> MKEVEVLMETKNTQSPQTPLVEPVTERTKLQEHTIFTQLKKNIPKTRYNRDYMLSMANIPERIINVGVIGPLHSGKTSLMDLLVIDSHKRIPDMSKNVELGWKPLRYLDNLKQEIDRGLSIKLNGSTLLCTDLESKSRMINFLDAPGHVNFMDETAVALAASDLVLIVIDVVEGVTFVVEQLIKQSIKNNVAMCFVINKLDRLILDLKLPPMDAYLKLNHIIANINSFTKGNVFSPIDNNIIFASTKLGFTFTIKEFVSYYYAHSIPSSKIDDFTTRLWGSVYYHKGNFRTKPFENVEKYPTFVEFILIPLYKIFSYALSMEKDKLKNLLRSNFRVNLSQEALQYDPQPFLKHVLQLIFRQQTGLVDAITRCYQPFELFDNKTAHLSIPGKSTPEGTLWAHVLKTVDYGGAEWSLVRIYSGLLKRGDTVRILDTSQSESRQKRQLHDISKTETSNEDEDEDDETPSCEVEEIGLLGGRYVYPVHEAHKGQIVLIKGISSAYIKSATLYSVKSKEDMKQLKFFKPLDYITEAVFKIVLQPLLPRELPKLLDALNKISKYYPGVIIKVEESGEHVILGNGELYMDCLLYDLRASYAKIEIKISDPLTVFSESCSNESFASIPVSNSISRLGEENLPGLSISVAAEPMDSKMIQDLSRNTLGKGQNCLDIDGIMDNPRKLSKILRTEYGWDSLASRNVWSFYNGNVLINDTLPDEISPELLSKYKEQIIQGFYWAVKEGPLAEEPIYGVQYKLLSISVPSDVNIDVMKSQIIPLMKKACYVGLLTAIPILLEPIYEVDITVHAPLLPIVEELMKKRRGSRIYKTIKVAGTPLLEVRGQVPVIESAGFETDLRLSTNGLGMCQLYFWHKIWRKVPGDVLDKDAFIPKLKPAPINSLSRDFVMKTRRRKGISTGGFMSNDGPTLEKYISAELYAQLRENGLVPWSHP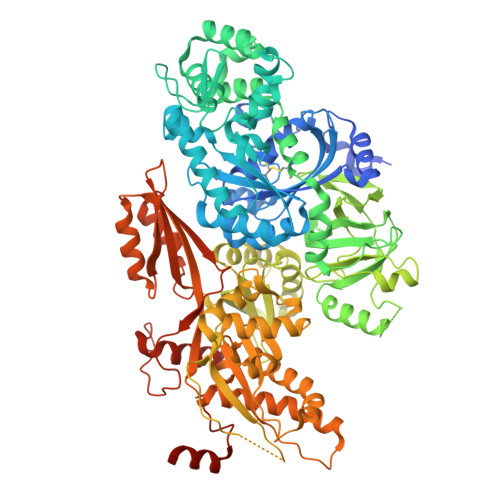QFEK>[4x]MSSSYDEASLAPEETTDSFWEVGNYKRTVKRIDDGHRLCNDLMNCVQERAKIEKAYGQQLTDWAKRWRQLIEKGPQYGSLERAWGAIMTEADKVSELHQEVKNNLLNEDLEKVKNWQKDAYHKQIMGGFKETKEAEDGFRKAQKPWAKKMKELEAAKKAYHLACKEEKLAMTREMNSKTEQSVTPEQQKKLQDKVDKCKQDVQKTQEKYEKVLEDVGKTTPQYMENMEQVFEQCQQFEEKRLVFLKEVLL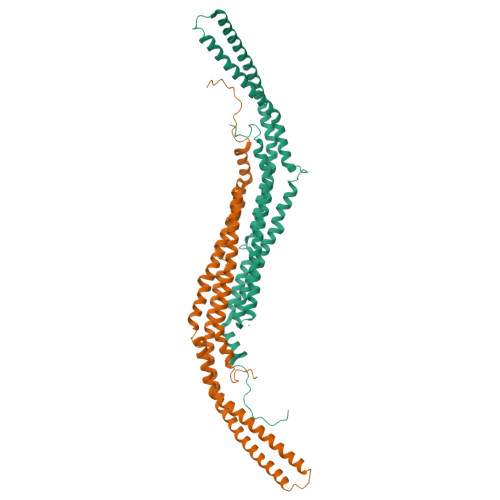DIKRHLNLAENSSYIHVYRELEQAIRGADAQEDLRWFRSTSGPGMPMNWPQFEEWNPD>SFSMPESGKAAFWDTKGDNFIHDPSIIKEGNTWYTFGTGLGTGLRVIKSTDGRNWSAAPSIFPTPLSWWKMYVPNHEPHQWAPDISYYNGRYWLYYSVSSFGSNTSAIGLASTDRISSGQWRDDGLVIRSTSGDQFNAIDPDLVIDKDGNPWLSFGSFWSGIKLTRLDKNTMKPTGSLYSIASRPNNGGAVEAPNITY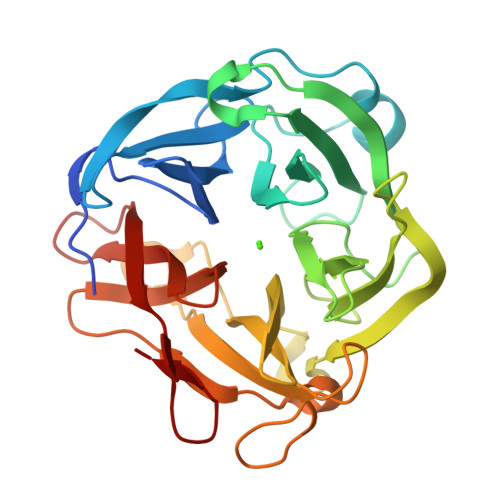KDGYYYLFVSFDSCCKGVDSTYKIAYGRSTSITGPYYDKSGKNMMNGGGTILDSGNDRWKGPGHQDVLNNSILVRHAYDALDNGVSKLLINDLYWDSQGWPTY[4x]The Klebsiella jumbo myophage ϕKp24 displays an unusually complex arrangement of tail fibers interacting with a host cell. We observe the tail fibers are branched and rearranged dramatically upon cell surface attachment. This complex configuration involves fourteen putative tail fibers with depolymerase activity that provide ϕKp24 with the ability to infect a broad panel of capsular polysaccharide (CPS) types of Klebsiella pneumoniae. In this study, we combine cryo-electron microscopy methods, protein structure prediction methods, molecular simulations, microbiological and machine learning approaches to explore the capsid, tail, and tail fibers of ϕKp24. We determine the structure of the capsid and tail at 4.1 Å and 3.0 Å resolution.

After classification, polishing, and 3D refinement, the tail structure (EMD-14357) in its extended conformation was determined to a resolution of 3.0 Å in Relion13. The full-length sheath protein is composed of outer and central sheath components. The outer sheath component (light blue) is located at the tip of the sheath monomer, pointing outwards. The central sheath component (orange, and dark blue) consists of the C-terminal domain, N-terminal domain, and two long extensions. The central sheath is essential in sheath assembly and contraction. To facilitate the interactions between tail sheath proteins in the tail, the two long extensions from the central sheath (the N-terminal extension, residues M1—S21; the C-terminal extension, residues A667—G689) can connect to the C-terminal domains of two adjacent gp118 proteins located in the ring below. Additionally, the C-terminal domain can connect with two adjacent sheath proteins located in the upper ring. Thus, three sheath proteins from two different layers link together within a so-called ridge. Furthermore, the structure solved here suggests that the subunit-connecting extensions (C-terminal extension) of the sheath protein gp118 function as hinges during contraction, with the central sheath of gp118 likely maintaining its structure.

>MSEQITGSTPRIYYRGTKDSSVTRSTGSTTTLPLHRPLIMFFGQKGPTVPTWIDPVKFEDIYGSETTNLSGVYCTHSTPFIKEAIAAGNQFMALRLEPSDIPDVATLGLSVDWVKTKIDDYERNDDGTYKLDTNGDKIPLATQIDGIKFRFVLEKIETNESGVSQYKKRTAKAGTIGTEATPSTITPLADFRCRFKSSLGANTALRIWAPTINSAQAADADLQARIKSFLYRFQILTRADKASSPTIFETIYNEPSLSVGFGENLVDPQTEVVYDFVERIDSRYNDEDPSTYLMSPLDTPYLYQANIDSVLTAIQELEAPFDTVSADEDDLYQINLFGAQTVEGVPYHAVQILGVLDGGVTLTETATNYLQGGGDGTLGNDSFNAAAYAVLSNLSNNAAFNITNYARYPFNAFWDSGFDLKTKQTIPQLIGLRADTWIALSTQDISSDFNSNEEEESIALSLMSRVSAFPDSSDFGTPAFRGMIVGGAGYYTETTRKLPVPLTLDRFRAYCRYAGASDGVLKPEYAVDEGDARKVQVVKSINNLDKSWRVRRAQWNNNLVYVEDYDTNSQFYPGQQSFYSEQGSVLKAAIVGLCVANLNRFAFEAWRDLTGTQKLTDDQLIERSDDAVSTRGTGAFDDRLIFTPHSEITQADKERGYSWSMRIDFGANAFRTVMDMSSVAYTREELANG[18x]> APTIPQGQGKVTFNNTVVDAPCSISQKSADQSIDFGQLSKSFLEAGGVSKPMDLDIELVNCDITAFKGGNGAKKGTVKLAFTGPIVNGHSDELDTNGGTGLAIVVQGAGKNVVFDGSEGDANTLKDGENVLHYTAVVK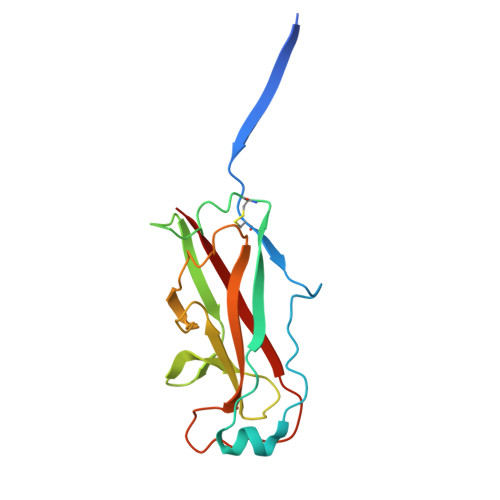KSSAVGAAVTEGAFSAVANFNLTYQ> MGSSHHHHHHENLYFQSNASKPRRTKLVFDDRNYSADHYLQEAKKLKHNADALSDRFEKAVYYLDAVVSFIECGNALEKNAQESKSPFPMYSETVDLIKYTMKLKNYLAPDATAADKRLTVLCLRCESLLYLRLFKLKKENALKYSKTLTEHLKNSYNNSQAPSPGLGSKAVGMPSPVSPKLSPG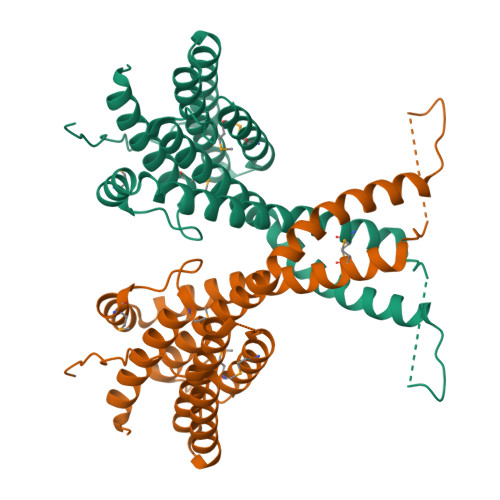NSGNYSSGASSASASGSSVTIPQKIHQMAASYVQVTSNFLYATEIWDQAEQLSKEQKEFFAELDKVMGPLIFNASIMTDLVRYTRQGLHWLRQDAKLIS The self-splicing group II introns are bacterial and organellar ancestors of the nuclear spliceosome and retro-transposable elements of pharmacological and biotechnological importance. Besides catalyzing their self-splicing, group II introns also act as mobile retroelements, thus crucially contributing to genetic diversity throughout evolution. Integrating enzymatic, crystallographic, and simulation studies, we demonstrate how these introns recognize small molecules through their conserved active site. These RNA-binding small molecules selectively inhibit the two steps of splicing by adopting distinctive poses at different stages of catalysis, and by preventing crucial active site conformational changes that are essential for splicing progression.

Using Oi5eD1-5, we first obtained a structure of the pre-catalytic state (the stage prior to the first step of splicing) in the presence of Ca2+, K+, and intronistat B at 4.0 Å resolution. The simulated-annealing electron density map generated by omitting the G1 at the 5’ splice junction demonstrates that in this structure the active site is occupied only by the reaction substrates, i.e. the 5’-splice junction and the reaction nucleophile.

> GUUAUGUGUGCCCGGCAUGGGUGCAGUCUAUAGGGUGAGAGUCCCGAACUGUGAAGGCAGAAGUAACAGUUAGCCUAACGCAAGGGUGUCCGUGGCGACAUGGAAUCUGAAGGAAGCGGACGGCAAACCUUCGGUCUGAGGAACACGAACUUCAUAUGAGGCUAGGUAUCAAUGGAUGAGUUUGCAUAACAAAACAAAGUCCUUUCUGCCAAAGUUGGUACAGAGUAAAUGAAGCAGAUUGAUGAAGGGAAAGACUGCAUUCUUACCCGGGGAGGUCUGGAAACAGAAGUCAGCAGAAGUCAUAGUACCCUGUUCGCAGGGGAAGGACGGAACAAGUAUGGCGUUCGCGCCUAAGCUUGAACCGCCGUAUACCGAACGGUACGUACGGUGGUGUGG> MEYEWKPDEQGLQQILQLLKESQSPDTTIQRTVQQKLEQLNQYPDFNNYLIFVLTKLKSEDEPTRSLSGLILKNNVKAHFQNFPNGVTDFIKSECLNNIGDSSPLIRATVGILITTIASKGELQNWPDLLPKLCS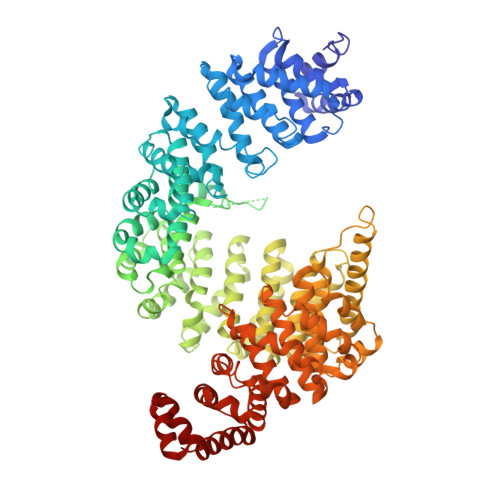LLDSEDYNTCEGAFGALQKICEDSAEILDSDVLDRPLNIMIPKFLQFFKHSSPKIRSHAVACVNQFIISRTQALMLHIDSFIENLFALAGDEEPEVRKNVCRALVMLLEVRMDRLLPHMHNIVEYMLQRTQDQDENVALEACEFWLTLAEQPICKDVLVRHLPKLIPVLVNGMKYSDIDIILLKGDVEEDETIPDSEQDIRPRFHRSRTVAQQHDEDGIEEEDDDDDEIDDDDTISDWNLRKCSAAALDVLANVYRDELLPHILPLLKELLFHHEWVVKESGILVLGAIAEGCMQGMIPYLPELIPHLIQCLSDKKALVRSITCWTLSRYAHWVVSQPPDTYLKPLMTELLKRILDSNKRVQEAACSAFATLEEEACTELVPYLAYILDTLVFAFSKYQHKNLLILYDAIGTLADSVGHHLNKPEYIQMLMPPLIQKWNMLKDEDKDLFPLLECLSSVATALQSGFLPYCEPVYQRCVNLVQKTLAQAMLNNAQPDQYEAPDKDFMIVALDLLSGLAEGLGGNIEQLVARSNILTLMYQCMQDKMPEVRQSSFALLGDLTKACFQHVKPCIADFMPILGTNLNPEFISVCNNATWAIGEISIQMGIEMQPYIPMVLHQLVEIINRPNTPKTLLENTAITIGRLGYVCPQEVAPMLQQFIRPWCTSLRNIRDNEEKDSAFRGICTMISVNPSGVIQDFIFFCDAVASWINPKDDLRDMFCKILHGFKNQVGDENWRRFSDQFPLPLKERLAAFYGV;> YSNQQSGYGKVSRRGGHQNSYKPY> DLKTEWPELVGKSVEEAKKVILQDKPEAQIIVLPVGTIVTMEYRIDRVRLFVDK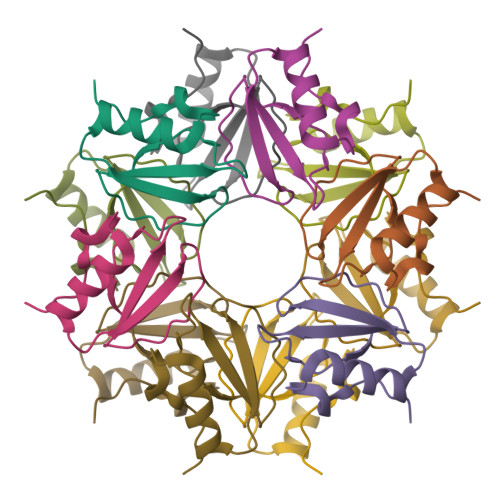LDNIAEVPRVG NALCN channel mediates sodium leak currents and is important for maintaining proper resting membrane potential. The functional NALCN channel is a hetero-tetrameric channelosome that is composed of NALCN, FAM155, UNC79, and UNC80 proteins, with a total molecular weight of 920 kDa1. NALCN protein is the pore-forming subunit of the complex and shares sequence and structural homology with eukaryotic voltage-gated sodium channels (NaV) and calcium channels (CaV). UNC79 and UNC80 facilitate robust currents of NALCN in a heterologous expression system, such as HEK293T cells or Xenopus oocyte.

Further extensive signal subtraction and focused refinements resolved five overlapping structural fragments at 2.9–3.7 Å resolution. Our final model encompasses 1346 out of 1738 residues of NALCN, 173 out of 467 residues of FAM155A, 1528 out of 2654 residues of UNC79, and 1711 out of 3326 residues of UNC80. The NALCN-FAM155A subcomplex sits above the central joint of the UNC79-UNC80 heterodimer to form an asymmetric quaternary complex occupying 200 Å × 315 Å × 145 Å 3D space. UNC79 and UNC80 interact in a head-to-tail fashion to form a plier-shape complex, akin to the infinity symbol “∞”. UNC79 and UNC80 interact through three regions: head, joint, and tail. We observed one C3H-type zinc finger between α26 and α27 of 80-UHD-M, and another C3H-type zinc finger between α46 and α47 of 79-UHD-M. NALCN interacts with UNC79-UNC80 heterodimer through three cytosolic UNC-interacting motifs (UNIM-A, B, C), which all are on loop regions of NALCN. UNIM-A has a short β hairpin structure which is inserted into a hydrophobic crevice formed between α48-α50 of UNC79. UNIM-B interacts with 80-UHD-M and 80-UCD2. Therefore, our structural observation and modeling study suggest that the binding of UNIM-C of NALCN DII-III linker to the UNC79-UNC80 heterodimer in the quaternary complex would prevent the binding of its neighboring CIH in the CIH-binding pocket of NALCN CTD, likely through spacial constrain, and UMIM-C-5A mutations would disrupt the binding of UNIM-C to UNC79-UNC80 and would release the constrain of UNIM-C on CIH to allow it to re-bind to NALCN CTD.

> MSTKAEQFASKIRYLQEYHNRVLHNIYPVPSGTDIANTLKYFSQTLLSVLRDAPSERGPQSRDAQLSDYPSLDYQGLYVTLVTLLDLVPLLQHGQHDLGQSIFYTTTCLLPFLNDDVLSTLPYTMISTLATFPPFLHKDIIEYLSTSFLPMAILGSSGREGVPAHVNLSASSMLMIAMQYTSNPVYHCQLLECLMKYKQEVWKDLLYVIAYGPSQVKPPAVQMLFHYWPNLKPPGAISEYRGLQYTAWNPIHCQHIECHNAINKPAVKMCIDPSLSVALGDKPPPLYLCEECSERISGDHSEWLIDVLLPQAEISAICQKKNCSSHVRRAVVTCFSAGCCGRHGNRPVRYCKRCHSNHHSNEVGATAETHLYQTSPPPINTRECGAEELVCAVEAVISLLKEAEFHAEQREHELNRRRQLGLSSSHHSLDNTDFDNKDDDKHDQRLLSQFGIWFLVSLCTPSENTPTESLARLVAMVFQWFHSTAYMMDDEVGSLVEKLKPQFVTKWLKTVCDVRFDVMVMCLLPKPMEFARVGGYWDKSCSTVTQLKEGLNRILCLIPYNVISQSVWECIMPEWLEAIRTEVPDNQLKEFREVLSKMFDIELCPLPFSMEEMFGFISCRFTGYPSTVQEQALLWLHVLSELDITVPLQLLISMFSDGVNSVKELANQRKSRANELAGNLASRRVSVASDPGRRGQHNTLSPFHSPFQSPFRSPMRSPFRSPFKNFGHPGGRTIDFDCEDDDMNLNCFILMFDLLLKQMELQDDGITMGLEHSLSKDIISIINNVFQAPWGGSHSCQKDKKATECNLCQSSILCYQLACELLERLAPKEESRLVEPTDSLEDSLLSSRPEFILGPEGEEEENPAAKHGENPGNRTVPSEHAAIKNDTERKFCYQQLPVTLRLIYTIFQEMAKFEEPDILFNMLNCLKILCLHGECLYTARKDHPQFLAYIQDHMLIASLWRVVKSEFSQLSSLAVPLLLHALSLPHGADIFWTIINGNFNSKDWKMRFEAVEKVAVICRFLDIHSVTKNHLLKYSLAHAFCCFLTAVEDVNPAVATRAGLLLDTIKRPALQGLCLCLDFQFDTVVKDRPTILSKLLLLHFLKQDIPALSWEFFVNRFETLSLEAQLHLDCNKEFPFPTTITAVRTNVANLSDAALWKIKRARFARNRQKSVRSLRDSVKGPAESKRALSLPETLTSKIPVRLTRHEQSAPALGGTPEQTPGQQSPENDNTIKDLLPEDAGIDHQTVHQLITVLMKFMARDESSAESDISSAKAFNTVKRHLYVLLGYDQQEGCFMIAPQKMRLSTCFNAFIAGIAQVMDYNINLGKHLLPLVVQVLKYCSCPQLRHYFQQPPRCSLWSLKPHIRQMWLKALLVILYKYPYRDCDVSKTLLHLIHITVNTLNAQYHSCKPHATAGPLYTDNSNISRYSEKEKEEDSVFDESDIHDTPTGPCNKESQTFFARLKRIGGSRMVKGQPVGMNVQRSEIELAEYRETGALQDSVLHCVREESIQKKKLRSLKQKSLDIGNADSLLFTLDEHRRKSCIDRCDIDKPPAQAAYISQRQNDHHGRSRQNSATRPDNTEIPKNPGTEGFQEIRRPVIPEVRLNCMETFEVRVDSPGKPAPREDLDLIDLSSDSTSGPEKHSILSTSDSDSLVFEPLPPLRIVESDEEEEMMNQGNGGALGNNAASSPSIPSQPSVLSLSTTPLVQVSVEDCSKDFSSKDSGNHQSASNEDSTIAALDDLTDSEELSKSEELREFASGSPLTLKQKRDLLQKSSAVPEMSVDYNPEPSPAEEKPGQTPTSGVKTVLLKVPEDGENLIESEKPNTSAESDTEQNPERKVEEDGAEESEFKIQIVPRQRKQRKIAVSAIQREYLDISFNILDKLGEQKDPDPSAKGLSTLEMPRESSSAPTLEAGAPETSSHSSISTQYRQMKRGSLGVLTMSQLMKRQLEHQSSAPHNISSWDTEQIQPGKRQCNVPMCLNPDLEGQPLRTRGATKSSLLSAPSIASMFVPAPEEFTEEQPTVMADKCHDCGAILEEYDEETLGLAIVVLSTFIHLSPDLAAPLLLDIMQSVGRLASSTTFSNQAESMMVPGNAAGVAKQFLRCIFHQLAPNGIFPQLFQSAIKDGTFLRTLATSLMDFNELSSIAALSQLLEGLNNKKNLPAGGAMIRCLENIATFMEALPMDSPSSLWTTISNQFQTFFAKLPCVLPLKCSLDSSLRIMICLLKIPSTNATRSLLEPFSKLLSFVIQNAVFTLAYLVELCGLCYRAFTKERDKFYLSRSVVLELLQALKLKSPLPDTNLLLLVQFICADAGTKLAESTILSKQMIASVPGCGTAAMECIRQYVSEVLEFMADMHTLTKLKSHMKTCSQPLHEDTFGGHLKVGLAQIAAMEISRGNHRDNKAVIRYLPWLYHPPSAMQQGPKEFIECVSHIRLLSWLLLGSLTHNAVCPNASSPCLPIPLDAGSHIADHLIVILIGFPEQSKTCVLHMCSLFHAFIFAQLWTVYCEQSAVATNVQNQNEFSFTAILTALEFWSRVTPSILQLMAHNKVMVEMVCLHVISLMEALQECNSTIFVKLIPMWLPMIQSNTKHLSAGLQLRLQAIQNNVNHHSLRTLPGSGQSSAGLAALRKWLQCTQFKMAQVEIQSSEAASQFYPL;> MVKRKSSEGQEQDGGRGIPLPIQTFLWRQTSAFLRPKLGKQYEASCVSFERVLVENKLHGLSPALSEAIQSISRWELVQAALPHVLHCTATLLSNRNKLGHQDKLGVAETKLLHTLHWMLLEAPQDCNNDQFGGTDRGSSWGGSSSAFIHQIENQGSPGQPCRSSSHDEEENNRRKTFQNSMATVELFVFLFAPLVHRIKESDLTFRLASGLVIWQPMWEHRQPEVSGFTALVKPIRNIITAKRSSPINSQSQTCESPNQDTRQQGEGLQVVSEALQSDSISPKATISGCHQGNSFDGSLSSQTSQERGPSHSRASLVIPPCQRSRYATYFDVAVLRCLLQPHWSEEGTQWSLMYYLQRLRHMLEEKPEKTPDPDIPLLPRPRSSSMVAAAPSLVNTHKTQDLTMKCNEEEKSLSPEAFSKVSLTNLRRSAVPDLSSDLGMNIFKKFKSRKEDRERKGSIPFHHTGKRRPRRMGVPFLLHEDHLDVSPTRSTFSFGSFSGLGEDRRGIEKGGWQTTILGKLTRRGSSDAATEMESLSARHSHSHHTLVSDLPDHSNSHGENTVKEVRSQISTITVATFNTTLASFNVGYADFFSEHMRKLCSQVPIPEMPHEPLACANLPRSLTDSCINYSYLEDTEHIDGTNNFVHKNGMLDLSVVLKAVYLVLNHDISSRICDVALNIVECLLQLGVVPCVEKNRKKSENKENESVEKRPSEGAFQFKGVSSSSTSGFGAPSASGAGDGGGEEGGGGDGGGGGGGGDGGGGGGGGGGPYEKNEKNQEKDDNIPVSNHRLALTMLIKIVKSLGCAYGCGEGHRGLSGDRLRHQVFRENAQNCLTKLYKLDKIQFRQTMRDYVNKDSLNNVVDFLHALLGFCMEPVTDNKAGFGNNFTTVDNKSTAQNVEGIIVGAMFKSLITRCASTTHELHSPENLGLYCDIRQLVQFIKEAHGNVFRRVALSALLDSAEKLAPGKKVEENGQESKPVGSKRSEAGSIADKGQVSSAPEECRSFMSGRPSQTPEHDEPMQGGNLGRKDFWRKMFKSQSAASDTSSQSEQDTSECTTAHSGNTSDRRARSRSRRISLRKKLKLPIGNWLKRSSLSGLADGVEDLLDISSVDRLSFIRQSSKVKFTSAVKLSEGGPGSGMENGREEEENFFKRLGCHSFDDHLSPNQDGGKSKNVVNLGAIRQGMKRFQFLLNCCEPGTIPDASILAAALDLEAPVVARAALFLECARFVHRCNRGNWPEWMKGHHVNITKKGLSRGRSPTVGNKRNQKLQWSAAKLFYQWGDAIGIRLNELCHGESESPANLLGLIYDEETKRRLRKEDEEEDFLDDSTVNPSKCGCPFALKMAACQLLLEITTFLRETFSCLPRPRTEPLVDLESCRLRLDPELDRHRYERKISFAGVLDENEDSKDSLHSSSHTIKSDAGAEEKKVPSRKIRIGGSRLLQIKGTRSFQVKKGGSLSSIRRVGSLKSSKLSRQDSESEAEELQLSQSRDTVTDLEGSPWSASEPSIEPEGLSNAGTEENYHRNMSWLHVMILLCNQQSFICTHVDYCHPHCYLHHSRSCARLVRAIKLLYGDSVDSLRESNHISNVALRGKKQKECSDKSCLRTPSLKKRVSDVNLEGKKDSGMLKYIRFQVMSLSPAPLSLLIKAAPILTEEMYGDIQPAAWELLLSMDEHMAGAAAAMFLLCAVKVPDAVSDMLMSEFHHAETVQRLNAVLKFHTLWRFRYQVWPRMEEGAQQIFKIPPPSINFTLPSPVLGMPSVPMFDPPWVPQCSGSVQDPINEDQSKSFSARAVSRSHQRAEHILKNLQQEEEKKRLGREASLITAIPITQEACYEPTCTPNSEPEEEEEVANLTSRRLSVSPSCTSSTSHRNYSFRRGSVWSVRSAVSAEDEEHATEHTPNHHVPQPPQAVFPACICAAVLPIVHLMEDGEVREDGVAVSAVAQQVLWNCLIEDPSTVLRHFLEKLTISNRQDELMYMLRKLLLNIGDFPAQTSHILFNYLVGLIMYFVRTPCEWGMDAISATLTFLWEVVGYVEGLFFKDLKQTMKKEQCEVKLLVTASMPGTKTLVVHGQNECDIPTQLPVHEDTQFEALLKECLEFFNIPESQSTHYFLMDKRWNLIHYNKTYVRDIYPFRRSVSPQLNLVHMHPEKGQELIQKQVFTRKLEEVGRVLFLISLTQKIPTAHKQSHVSMLQEDLLRLPSFPRSAIDAEFSLFSDPQAGKELFGLDTLQKSLWIQLLEEMFLGMPSEFPWGDEIMLFLNVFNGALILHPEDSALLRQYAATVINTAVHFNHLFSLSGYQWILPTMLQVYSDYESNPQLRRAIEFACHQFYILHRKPFVLQLFASVAPLLEFPDAANTGSSKGVSAQCLFDLLQSLEGETTDILDILELVKAEKPLKSLDFCYGNEDLTFSISEAIKLCVTVVAYAPESFRSLQMLMVLEALVPCYLQKMKRQTSQVETVPAAREEIAATAALATSLQALLYSVEVLTRPMTAPQMSRSDQGHKGTTTANHTMSSGVNTRYPEQGAKLHFIRENLHLLEEGQGLPREELDERISREEFRRPRESLLNICTEFYKHCGPRLKILQNLAGEPRVTALELLDVKSHMRLAEIAHSLLKLAPYDTQTMESRGLRRYIMEMLPITDWSAEAVRPALILILKRLDRMFNKIHKMPTLRRQVEWEPASSLIEGVCLTLQRQPIISFLPHLRSLINVCVNLVMGVVGPSSVADGLPLLHLSPYLSPPLPFSTAVVRLVALQIQALKEDFPLSHVISPFTNQERREGMLLNLLIPFVLTVGSGSKDSPWLEQPEVQLLLQTVINVLLPPRIISTSRSKNFMLESSPAHCSTPGDAGKDLRKEGLAESTSQAAYLALKVILVCFERQLGSQWYWLSLQVKEMALRKVGGLALWDFLDFIVRTRIPIFVLLRPFIQCKLLAQPAENHEELSARQHISDQLERRFIPRPLCKSSLIAEFNSELKILKEAVHSGSAYQGKTSISTVGTSTSAYRLSLATMSRSNTGTGTVWEQDSEPSQQASQDTLSRTDEEDEENDSVSMPSVVSEQEACLLSTIGRRRFSSHVSSMSAPQAEVGMLPSQSEPNVLDDSQGLAAEGSLSRVASIQSEPGQQNVLLQQPLGRKRGLRQLRRPLLSRQKTQTEPRNRHGARLSTTRRSIQPKTKPSVDQKRSVTFIEAQPEPTAAPTDIFPATGQPQSCSPGRARKPEGTEKPVLTSSPAIIIADLHSLSPKQSEPLLAEEGEKKEDEEIQGATAHCPLSTQLSDPDDFTGLETSSLLQHGDTVLHISEENGTENPLLSSQFTFTPPELGDTDSALDESHV;> MLKRKQSSRVEAQPVTDFGPDESLSDNADILWINKPWVHSLLRICAIISVISVCMNTPMTFEHYPPLQYVTFTLDTLLMFLYTAEMIAKMHIRGIVKGDSSYVKDRWCVFDGFMVFCLWVSLVLQVFEIADIVDQMSPWGMLRIPRPLIMIRAFRIYFRFELPRTRITNILKRSGEQIWSVSIFLLFFLLLYGILGVQMFGTFTYHCVVNDTKPGNVTWNSLAIPDTHCSPELEEGYQCPPGFKCMDLEDLGLSRQELGYSGFNEIGTSIFTVYEASSQEGWVFLMYRAIDSFPRWRSYFYFITLIFFLAWLVKNVFIAVIIETFAEIRVQFQQMWGTRSSTTSTATTQMFHEDAAGGWQLVAVDVNKPQGRAPACLQKMMRSSVFHMFILSMVTVDVIVAASNYYKGENFRRQYDEFYLAEVAFTVLFDLEALLKIWCLGFTGYISSSLHKFELLLVIGTTLHVYPDLYHSQFTYFQVLRVVRLIKISPALEDFVYKIFGPGKKLGSLVVFTASLLIVMSAISLQMFCFVEELDRFTTFPRAFMSMFQILTQEGWVDVMDQTLNAVGHMWAPLVAIYFILYHLFATLILLSLFVAVILDNLELDEDLKKLKQLKQSEANADTKEKLPLRLRIFEKFPNRPQMVKISKLPSDFTVPKIRESFMKQFIDRQQQDTCCLFRILPSTSSSSCDNPKRPTVEDNKYIDQKLRKSVFSIRARNLLEKETAVTKILRACTRQRMLSGSFEGQPAKERSILSVQHHIRQERRSLRHGSNSQRISRGKSLETLTQDHSNTVRYRNAQREDSEIKMIQEKKEQAEMKRKVQEEELRENHPYFDKPLFIVGREHRFRNFCRVVVRARFNASKTDPVTGAVKNTKYHQLYDLLGLVTYLDWVMITVTICSCISMMFESPFRRVMHAPTLQIAEYVFVIFMSIELNLKIMADGLFFTPTAVIRDFGGVMDIFIYLVSLIFLCWMPQNVPAESGAQLLMVLRCLRPLRIFKLVPQMRKVVRELFSGFKEIFLVSILLLTLMLVFASFGVQLFAGKLAKCNDPNIIRREDCNGIFRINVSVSKNLNLKLRPGEKKPGFWVPRVWANPRNFNFDNVGNAMLALFEVLSLKGWVEVRDVIIHRVGPIHGIYIHVFVFLGCMIGLTLFVGVVIANFNENKGTALLTVDQRRWEDLKSRLKIAQPLHLPPRPDNDGFRAKMYDITQHPFFKRTIALLVLAQSVLLSVKWDVEDPVTVPLATMSVVFTFIFVLEVTMKIIAMSPAGFWQSRRNRYDLLVTSLGVVWVVLHFALLNAYTYMMGACVIVFRFFSICGKHVTLKMLLLTVVVSMYKSFFIIVGMFLLLLCYAFAGVVLFGTVKYGENINRHANFSSAGKAITVLFRIVTGEDWNKIMHDCMVQPPFCTPDEFTYWATDCGNYAGALMYFCSFYVIIAYIMLNLLVAIIVENFSLFYSTEEDQLLSYNDLRHFQIIWNMVDDKREGVIPTFRVKFLLRLLRGRLEVDLDKDKLLFKHMCYEMERLHNGGDVTFHDVLSMLSYRSVDIRKSLQLEELLAREQLEYTIEEEVAKQTIRMWLKKCLKRIRAKQQQSCSIIHSLRESQQQELSRFLNPPSIETTQPSEDTNANSQDHNTQPESSSQQQLLSPTLSDRGGSRQDAADTGKPQRKIGQWRLPSAPKPISHSVSSVNLRFGGRTTMKSVVCKMNPMPDTASCGSEVKKWWTRQLTVESDESGDDLLDI;> MTRGAWMCRQYDDGLKIWLAAPRENEKPFIDSERAQKWRLSLASLLFFTVLLSDHLWFCAEAKLTRTRDKEHHQQQQQQQQQQQQQQQQQQQQQQRQQQRQRQQQRQRQQEPSWPALLASMGESSPAAQAHRLLSASSSPTLPPSPGGGGGSKGNRGKNNRSRALFLGNSAKPVWRLETCYPQGASSGQCFTVESADAVCARNWSRGAAAGEEQSSRGSRPTPLWNLSDFYLSFCNSYTLWELFSGLSSPSTLNCSLDVVLTEGGEMTTCRQCIEAYQDYDHHAQEKYEEFESVLHKYLQSDEYSVKSCPEDCKIVYKAWLCSQYFEVTQFNCRKTIPCKQYCLEVQTRCPFILPDNDEVIYGGLSSFICTGLYETFLTNDEPECCDIRSEEQTAPRPKGTVDRRDSCPRTSLTVSSATRLCPGRLKLCVLVLILLHTVLTASAAQNSTGLGLGGLPTLEDNSTRED>MSLVLNDLLICCRQLEHDRATERKKEVEKFKRLIRDPETIKHLDRHSDSKQGKYLNWDAVFRFLQKYIQKETECLRIAKPNVSASTQASRQKKMQEISSLVKYFIKCANRRAPRLKCQELLNYIMDTVKDSSNGAIYGADCSNILLKDILSVRKYWCEISQQQWLELFSVYFRLYLKPSQDVHRVLVARIIHAVTKGCCSQTDGLNSKFLDFFSKAIQCARQEKSSSGLNHILAALTIFLKTLAVNFRIRVCELGDEILPTLLYIWTQHRLNDSLKEVIIELFQLQIYIHHPKGAKTQEKGAYESTKWRSILYNLYDLLVNEISHIGSRGKYSSGFRNIAVKENLIELMADICHQVFNEDTRSLEISQSYTTTQRESSDYSVPCKRKKIELGWEVIKDHLQKSQNDFDLVPWLQIATQLISKYPASLPNCELSPLLMILSQLLPQQRHGERTPYVLRCLTEVALCQDKRSNLESSQKSDLLKLWNKIWCITFRGISSEQIQAENFGLLGAIIQGSLVEVDREFWKLFTGSACRPSCPAVCCLTLALTTSIVPGTVKMGIEQNMCEVNRSFSLKESIMKWLLFYQLEGDLENSTEVPPILHSNFPHLVLEKILVSLTMKNCKAAMNFFQSVPECEHHQKDKEELSFSEVEELFLQTTFDKMDFLTIVRECGIEKHQSSIGFSVHQNLKESLDRCLLGLSEQLLNNYSSEITNSETLVRCSRLLVGVLGCYCYMGVIAEEEAYKSELFQKAKSLMQCAGESITLFKNKTNEEFRIGSLRNMMQLCTRCLSNCTKKSPNKIASGFFLRLLTSKLMNDIADICKSLASFIKKPFDRGEVESMEDDTNGNLMEVEDQSSMNLFNDYPDSSVSDANEPGESQSTIGAINPLAEEYLSKQDLLFLDMLKFLCLCVTTAQTNTVSFRAAD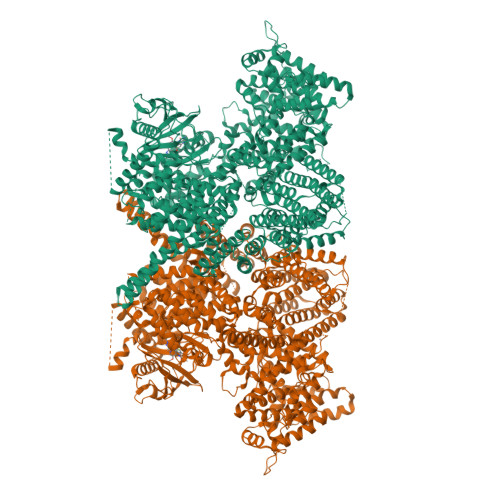IRRKLLMLIDSSTLEPTKSLHLHMYLMLLKELPGEEYPLPMEDVLELLKPLSNVCSLYRRDQDVCKTILNHVLHVVKNLGQSNMDSENTRDAQGQFLTVIGAFWHLTKERKYIFSVRMALVNCLKTLLEADPYSKWAILNVMGKDFPVNEVFTQFLADNHHQVRMLAAESINRLFQDTKGDSSRLLKALPLKLQQTAFENAYLKAQEGMREMSHSAENPETLDEIYNRKSVLLTLIAVVLSCSPICEKQALFALCKSVKENGLEPHLVKKVLEKVSETFGYRRLEDFMASHLDYLVLEWLNLQDTEYNLSSFPFILLNYTNIEDFYRSCYKVLIPHLVIRSHFDEVKSIANQIQEDWKSLLTDCFPKILVNILPYFAYEGTRDSGMAQQRETATKVYDMLKSENLLGKQIDHLFISNLPEIVVELLMTLHEPANSSASQSTDLCDFSGDLDPAPNPPHFPSHVIKATFAYISNCHKTKLKSILEILSKSPDSYQKILLAICEQAAETNNVYKKHRILKIYHLFVSLLLKDIKSGLGGAWAFVLRDVIYTLIHYINQRPSCIMDVSLRSFSLCCDLLSQVCQTAVTYCKDALENHLHVIVGTLIPLVYEQVEVQKQVLDLLKYLVIDNKDNENLYITIKLLDPFPDHVVFKDLRITQQKIKYSRGPFSLLEEINHFLSVSVYDALPLTRLEGLKDLRRQLELHKDQMVDIMRASQDNPQDGIMVKLVVNLLQLSKMAINHTGEKEVLEAVGSCLGEVGPIDFSTIAIQHSKDASYTKALKLFEDKELQWTFIMLTYLNNTLVEDCVKVRSAAVTCLKNILATKTGHSFWEIYKMTTDPMLAYLQPFRTSRKKFLEVPRFDKENPFEGLDDINLWIPLSENHDIWIKTLTCAFLDSGGTKCEILQLLKPMCEVKTDFCQTVLPYLIHDILLQDTNESWRNLLSTHVQGFFTSCLRHFSQTSRSTTPANLDSESEHFFRCCLDKKSQRTMLAVVDYMRRQKRPSSGTIFNDAFWLDLNYLEVAKVAQSCAAHFTALLYAEIYADKKSMDDQEKRSLAFEEGSQSTTISSLSEKSKEETGISLQDLLLEIYRSIGEPDSLYGCGGGKMLQPITRLRTYEHEAMWGKALVTYDLETAIPSSTRQAGIIQALQNLGLCHILSVYLKGLDYENKDWCPELEELHYQAAWRNMQWDHCTSVSKEVEGTSYHESLYNALQSLRDREFSTFYESLKYARVKEVEEMCKRSLESVYSLYPTLSRLQAIGELESIGELFSRSVTHRQLSEVYIKWQKHSQLLKDSDFSFQEPIMALRTVILEILMEKEMDNSQRECIKDILTKHLVELSILARTFKNTQLPERAIFQIKQYNSVSCGVSEWQLEEAQVFWAKKEQSLALSILKQMIKKLDASCAANNPSLKLTYTECLRVCGNWLAETCLENPAVIMQTYLEKAVEVAGNYDGESSDELRNGKMKAFLSLARFSDTQYQRIENYMKSSEFENKQALLKRAKEEVGLLREHKIQTNRYTVKVQRELELDELALRALKEDRKRFLCKAVENYINCLLSGEEHDMWVFRLCSLWLENSGVSEVNGMMKRDGMKIPTYKFLPLMYQLAARMGTKMMGGLGFHEVLNNLISRISMDHPHHTLFIILALANANRDEFLTKPEVARRSRITKNVPKQSSQLDEDRTEAANRIICTIRSRRPQMVRSVEALCDAYIILANLDATQWKTQRKGINIPADQPITKLKNLEDVVVPTMEIKVDHTGEYGNLVTIQSFKAEFRLAGGVNLPKIIDCVGSDGKERRQLVKGRDDLRQDAVMQQVFQMCNTLLQRNTETRKRKLTICTYKVVPLSQRSGVLEWCTGTVPIGEFLVNNEDGAHKRYRPNDFSAFQCQKKMMEVQKKSFEEKYEVFMDVCQNFQPVFRYFCMEKFLDPAIWFEKRLAYTRSVATSSIVGYILGLGDRHVQNILINEQSAELVHIDLGVAFEQGKILPTPETVPFRLTRDIVDGMGITGVEGVFRRCCEKTMEVMRNSQETLLTIVEVLLYDPLFDWTMNPLKALYLQQRPEDETELHPTLNADDQECKRNLSDIDQSFNKVAERVLMRLQEKLKGVEEGTVLSVGGQVNLLIQQAIDPKNLSRLFPGWKAWV[2x]> SNA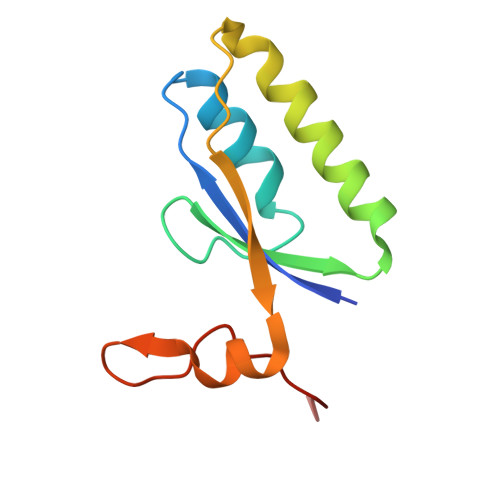MKHYLICFDVQHDKTRAKLSRLLEKYGPRVQGSVFEVSFKTPDRKRQLEYKIHQIIKQSNTEENNIRFYNLNKDTIKHSHDINGNPIAQLPAAIVL> IPEYVDWR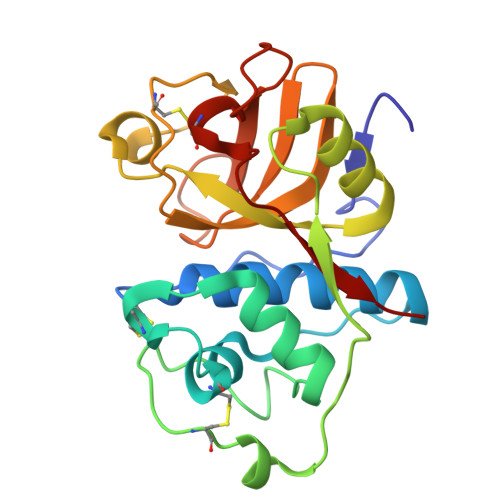QKGAVTPVKNQGSCGSCWAFSAVVTIEGIIKIRTGNLNEYSEQELLDCDRRSYGCNGGYPWSALQLVAQYGIHYRNTYPYEGVQRYCRSREKGPYAAKTDGVRQVQPYNEGALLYSIANQPVSVVLEAAGKDFQLYRGGIFVGPCGNKVDHAVAAVGYGPNYILIKNSWGTGWGENGYIRIKRGTGNSYGVCGLYTSSFYPVKN>QGHMSNFLAEQYERDRKAIINCCFSRPDHKTGEPPNNYITHVRIIEDSKFPSSRPPPDSKLENKKKRLLILSAKPNNAKLIQIHKARENSDGSFQIGRTWQLTELVRVEKDLEISEGFILTMSKKYYWETNSAKERTVFIKSLITLYIQTFEGHVPELVNWDLSLFYLDERSYQRAVITNRPGSVSPIKSPTSNFTTNTTQSVGSVPFSAPTERTRRSETESVNPVSTPASVEYHAGMK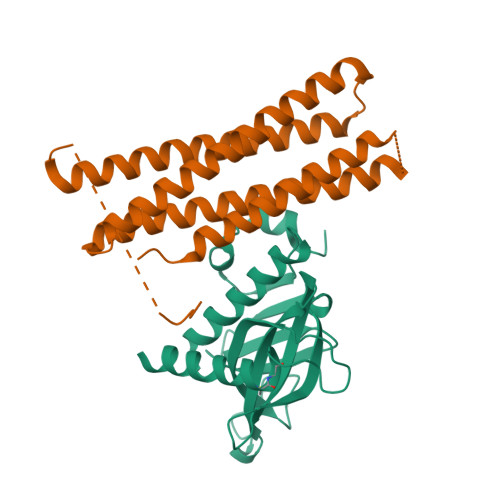SLNKAPYSSNS[2x];>GSHMMSNANPYENNNPYAENYEMQEDLNNAPTGHYEGSDDFVAFMNKINSINANLSRYENIINQIDAQHKDLLTQVSEEQEMELRRSLDDYISQATDLQYQLKADIKDAQRDGLHDSNKQAQAENCRQKFLKLIQDYRIIDSNYKEESKEQAKRQYTIIQPEATDEEVEAAINDVNGQQIFSQALLNANRRGEAKTALAEVQARHQELLKLEKTMAELTQLFNDMEELVIEQQENVDVIDKNVEDAQQDVEQGVGHTNKAVKSARKARKNKIRC[2x]>[4x]MGHHHHHHMRLQGKTALITGAARGIGLEFARAYIAEGARVALADINADAVRAAVESLGPQAVAVQMDVTRQDSIDAGFAEVIGTFGHLDILVNNAALFTAAPVEEVTRADYDRVMAVNMTGAFFCMQAAAKHMIARGKGGKIINMASQAGRRGEPLVAVYCASKAAVISMTQSAGLGLIRHGINVNAIAPGVVDGEHWDMVDEHFARFEGLKPG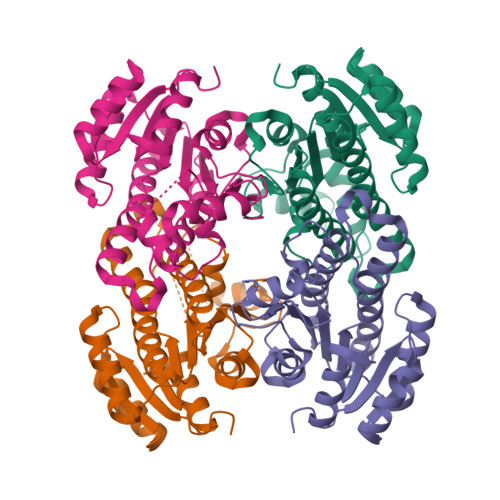EKKKLVGAAVPFGRMGVASDLTGMAIFLATAEAEYIVGQTFGVDGGNWLA Here it is shown which structural adaptations were introduced by directed evolution experiments that changed the catalytic properties of the Escherichia coli (E. coli) (S)-lactaldehyde reductase [EC 1.1.1.77]. This enzyme, referred to as FucO, is also known as an Fe2+, NAD+-dependent group-III alcohol de­hydrogenase and is involved in the catabolism of rare sugars in E. coli.

One route produced the single mutant L259V (dubbed variant D93). D93 displays features of a ‘generalist’ enzyme regarding substrate selectivity, retaining reasonable activities with compound 1 and its physiological substrate compound 2 and, in addition, being able to catalyze the reduction of the more bulky compound 3 with 13-fold improved catalytic efficiency (k cat /K M) compared with the wild-type. The mode of binding of NADH in the active site, including the nicotinamide moiety, is well defined by the electron density map, being the same in both structures. Here the crystal structures of DA1472 and its parent D93 (L259V) are reported, showing that these amino acid substitutions provide more space in the active site, though they do not cause changes in the main-chain conformation.

>MMANRMILNETAWFGRGAVGALTDEVKRRGYQKALIVTDKTLVQCGVVAKVTDKMDAAGLAWAIYDGVVPNPTITVVKEGLGVFQNSGADYLIAIGGGSPQDTCKAIGIISNNPEFADVRSLEGLSPTNKPSVPILAIPTTAGTAAEVTINYVITDEEKRRKFVCVDPHDIPQVAFIDADMMDGMPPALKAATGVDALTHAIEGYITRGAWALTDALHIKAIEIIAGALRGSVAGDKDAGEEMALGQYVAGMGFSNVGVGLVHGMAHPLGAFYNTPHGVANAILLPHVMRYNADFTGEKYRDIARVMGVKVEGMGLEEARNAAVEAVFALNRDVGIPPHLRDVGVRKEDIPALAQAALDDVCTGGNPREATLEDIVELYHTAWTSHHHHH[2x]> MKAETKSYKMDDGKTVDIPKDPKRIAVVAPTYAGGLKK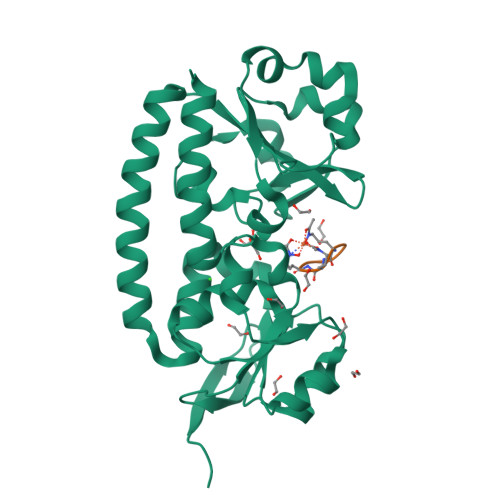LGANIVAVNQQVDQSKVLKDKFKGVTKIGDGDVEKVAKEKPDLIIVYSTDKDIKKYQKVAPTVVVDYNKHKYLEQQEMLGKIVGKEDKVKAWKKDWEETTAKDGKEIKKAIGQDATVSLFDEFDKKLYTYGDNWGRGGEVLYQAFGLKMQPEQQKLTAKAGWAEVKQEEIEKYAGDYIVSTSEGKPTPGYESTNMWKNLKATKEGHIVKVDAGTYWYNDPYTLDFMRKDLKEKLIKAAK;> GGGAAA> SHMASMKKKGSVVIVGRINLSGDTAYAQQTRGEEGCQETSQTGRDKNQVEGEVQIVSTATQTFLATSINGVLWTVYHGAGTRTIASPKGPVTQMYTNVDKDLVGWQAPQGSRSLTPCTCGSSDLYLVTRHADVIPVRRRGDSRGSLLSPRPISYLKGSSGGPL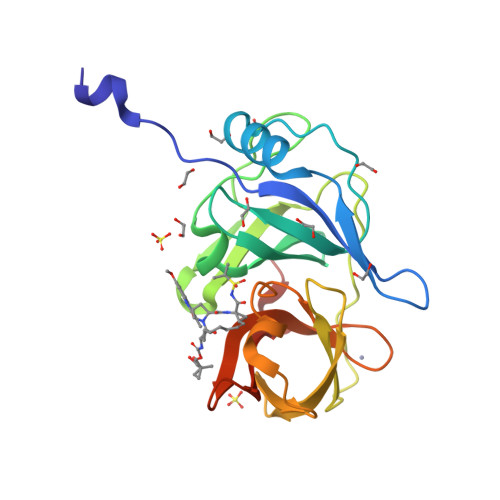LCPAGHAVGIFRAAVSTRGVAKAVAFIPVESLETTMRS> MHHHHHHKDEVALLATVTLVGVLLQAYFSLQVISA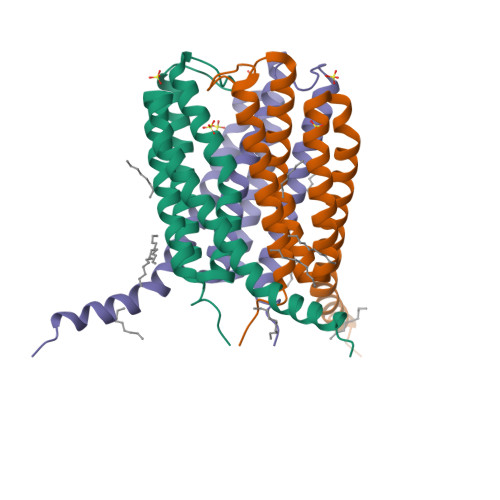RRAFHVSPPLTSGPPEFERVFRAQVNCSEYFPLFLATLWVAGIFFHEGAAALCGLFYLFARLRYFQGYARSAQLRLTPLYASARALWLLVAMAALGLLVHFLPGTLRTALFRWLQMLLPMA> SPQPLEQIKLSESQLSGRVGMIEMDLASGRTLTAWRADERFPMMSTFKVVLCGAVLARVDAGDEQLERKIHYRQQDLVEYSPVSEKHLADGMTVGELCAAAITMSDNSAANLLLATVGGPAGLTAFLRQIGDNVTRLDRWETELNEALPGDARDTTTPASMAATLRKLLTSQRLSARSQRQLLQWMVDDRVAGPLIRSVLPAGWFIADKTGAGERGARGIVALLGPNNKAERIVVIYLRDTPASMAERNQQIAGIG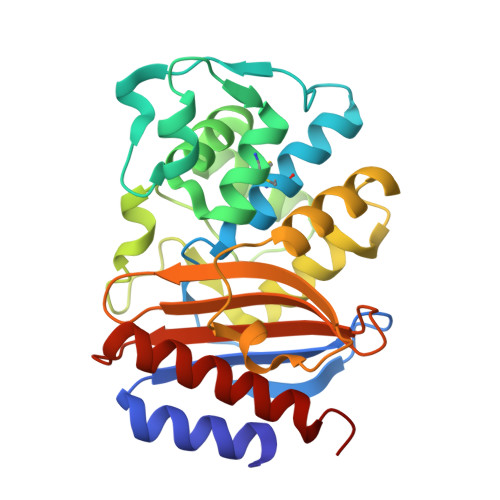AALIEHWQR> GPL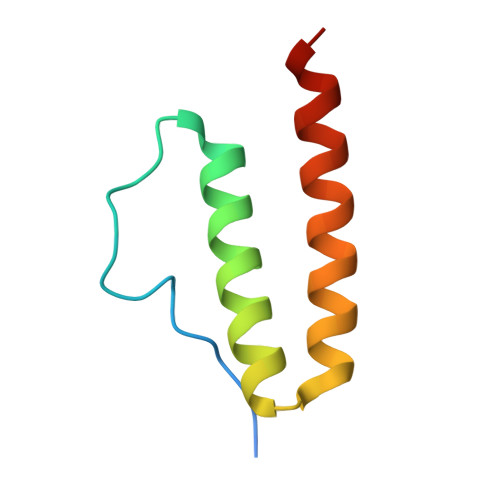GSAEGWLPLSGGQGQSEDSDPLLQQIHNITSFIRQAKAAGRMDEVRTLQENLRQLQDEYDQQQTEK>[4x]SPQSKSRKIAILGYRSVGKSSLTIQFVEGQFVDSYDPTIENTFTKLITVNGQEYHLQLVDTAGQDEYSIFPQTYSIDINGYILVYSVTSIKSFEVIKVIHGKLLDMVGKVQIPIMLVGN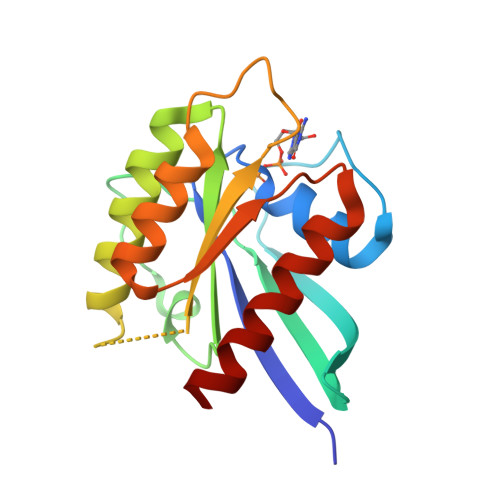KKDLHMERVISYEEGKALAESWNAAFLESSAKENQTAVDVFRRIILEAEKLE> EPTLVPTPPPELPTDCGGPFELWEPNTTFSSTNFPNSYPNLAFCVWILNAQKGKNIQLHFQEFDLENINDVVEIRDGEEADSLLLAVYTGPGPVKDVFSTTNRMTVLL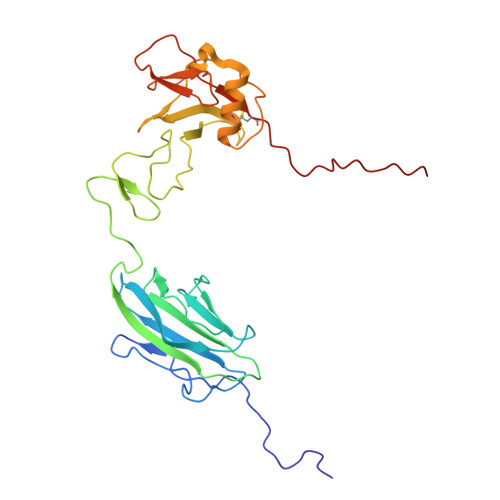ITADVLARGGFKANFTTGYHLGIPEPCKADHFQCKNGECVPLVNLCDGHLHCEDGSDEADCVRFFNGTTNNNGLVRFRIQSIWHTACAENWTTQISNDVCQLLGLGSGNSSKPIFPTDGGPFVKLNTAPDGHLILTPSQQCLQDSLIRLQCNHKSCGKKLAAQDITPK>MIINNLKLIRE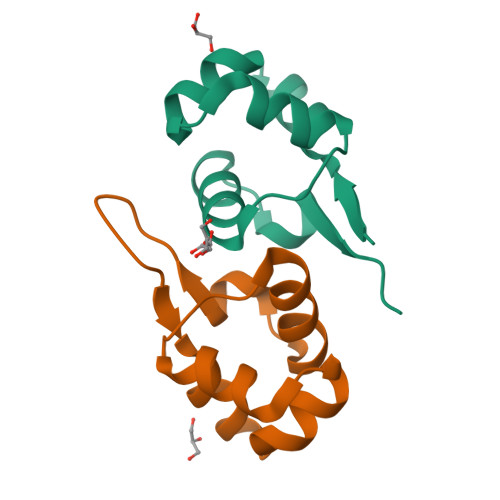KKKISQSELAALLEVSRQTINGIEKNKYNPSLQLALKIAYYLNTPLEDIFQWQPE[2x]>MGSDKIHHHHHHMKSLGRHLVAEFYECDREVLDNVQLIEQEMKQAAYESGA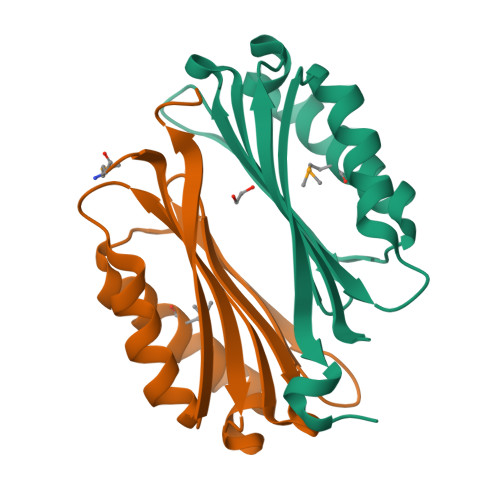TIVTSTFHRFLPYGVSGVVVISESHLTIHTWPEYGYAAIDLFTCGEDVDPWKAFEHLKKALKAKRVHVVEHERGRYDEIGIPEDSPHKAAV[2x]>MPGIMKNKKLLCSVCFLFAFMSALWGQNITVKGNVTSKTDGQPIIGASVVETTATTNGTITDFDGNFTLSVPVNSTLKITYIGYKPVTVKAAAIVNVLLEEDTQMVDEVVVTGYTTQRKADLTGAVSVVKVDEIQKQGENNPVKALQGRVPGMNITADGNPSGSATVRIRGIGTLNNNDPLYIIDGVPTKAGMHELNGNDIESIQVLKDAASASIYGSRAANGVIIITTKQGKKGQIKINFDASVSASMYQSKMNVLNTEQYGRAMWQAYVNDGENPNGNALGYAYNWGYNADGNPVLYGMTLSKYLDSKNTMPVADTDWFDEITRTGVIQQYNLSVSNGSEKGSSFFSLGYYKNLGVIKDTDFDRFSARMNSDYKLIDDILTIGQHFTLNRTSEVQAPGGIIETALDIPSAIPVYASDGSWGGPVGGWPDRRNPRAVLEYNKDNRYTYWRMFGDAYVNLTPFKGFNLRSTFGLDYANKQARYFTYPYQEGTQTNNGKSAVEAKQEHWTKWMWNAIATYQLEVGKHRGDVMIGMELNREDDSHFSGYKEDFSILTPDYMWPDAGSGTAQAYGAGEGYSLVSFFGKMNYSYADRYLLSLTLRRDGSSRFGKNHRYATFPSVSLGWRITQENFMKELTWLDDLKLRASWGQTGNQEISNLARYTIYAPNYGTTDSFGGQSYGTAYDITGSNGGGVLPSGFKRNQIGNDNIKWETTTQTNVGIDFSLFKQSLYGSLEYYYKKATDILTEMAGVGVLGEGGSRWINSGAMKNQGFEFNLGYRNKTAFGLTYDLNGNISTYRNEILELPETVAANGKFGGNGVKSVVGHTYGAQVGYIADGIFKSQDEVDNHATQEGAAVGRIRYRDIDHNGVIDERDQNWIYDPTPSFSYGLNIYLEYKNFDLTMFWQGVQGVDIISDVKKKSDFWSASNVGFLNKGTRLLNAWSPTNPNSDIPALTRSDTNNEQRVSTYFVENGSFLKLRNIQLGYTVPAVISKKMRMDRLRFYCSAQNLLTIKSKNFTGEDPENPNFSYPIPVNITFGLNIGF[2x];>[2x]MKKIIYIATIGITLLTTSCDDFLDRQVPQGIVTGDQIASPEYVDNLVISAYAIWATGDDINSSFSLWNYDVRSDDCYKGGSGTEDGGVFNALEISKGINTTDWNINDIWKRLYQCITRANTALQSLDQMDEKTYPLKNQRIAEMRFLRGHAHFMLKQLFKKIVIVNDENMEPDAYNELSNTTYTNDEQWQKIADDFQFAYDNLPEVQIEKGRPAQAAAAAYLAKTYLYKAYRQDGADNALTGINEEDLKQVVKYTDPLIMAKGGYGLETDYSMNFLPQYENGAESVWAIQYSINDGTYNGNLNWGMGLTTPQILGCCDFHKPSQNLVNAFKTDSQGKPLFSTYDNENYEVATDNVDPRLFHTVGMPGFPYKYNEGYIIQKNDDWSRSKGLYGYYVSLKENVDPDCDCLKKGSYWASSLNHIVIRYADVLLMRAEALIQLNDGRITDAISLINEVRSRAAGSTMLIFNYKEDYGVNFKVTPYDLKAYAQDEAMKMLKWERRVEFGMESSRFFDLVRWGEAKDVINAYYVTEASRCSIYKNAGFTENKNEYLPVPFEQISASNGNYTQNFGW;>MMKNMILPIAFTALIASMTACSDETDPILTQKNWDGTATYFQSSDEHGFSMYYKPQVGFVGAPMPFYDPVAKDFKVMYLQDYRPNPEATYHPIFGVATKDGATYESLGELISCGGRDEQDAAIGTGGTIYNPADKLYYTFYTGNKFKPSSDQNAQVVMVATSPDFKTWTKNRTFYLKGDTYGYDKNDFRDPFLFQTEDGVYHMLIATRKNGKGHIAEFTSADLKEWESAGTFMTMMWDRFYECPDVFKMGDWWYLIYSEQASFMRKVQYFKGRTLEDLKATTANDAGIWPDNREGMLDSRAFYAGKTASDGTNRYIWGWCPTRAGNDNGNVGDVEPEWAGNLVAQRLIQHEDGTLTLGVPDAIDRKYTSAQEVKVMAKDGNMIESGKTYTLGEGASVIFNRLKVHNKISFTVKTASNTDRFGISFVRGTDSASWYSIHVNADEGKANFEKDGDDAKYLFDNKFNIPADNEYRVTIYSDQSVCVTYINDQLSFTNRIYQMQKNPWSLCCYKGEITVSDVQVSTY[2x];>[2x]MKSIIKQLYTILLVTVACLTVTGCSDDFKSGLRLDGDVWVNSIRLDEYAGTVDYQNKAIVVGVPYDYDITRMVVTEMNLSEGAKASIAIGETIDFSLPVSLTVKNGDVQMSYTITVKRDEAKILTFKLNDTYVGKVDQLSKTISVVVPLTVDITQLKGTFTVTDGATVTPASGSIQDFTNPVTYTATYRSAVTPYVVTVTQGNVIPTAFVGTASSVSLLTSPEEKAAAQWMMDNVSMSEYISFKDVVDGKVDLGKYTAIWWHFHADNGDNPPLPDDAKAAAEKFKVYYQNGGNLLLTRYATFYIANLGIAKDERVPNNSWGGNEDSPEITSAPWSFLITGSESHPLFQDLRWKDGDKSTVYTCDAGYAITNSTAQWHIGTDWGGYDDLNAWRNLTGGIDLAHGGDGAVVIAEFEPRSNSGRTLCIGSGCYDWYGKGVDASADYYHYNVEQMTLNAINYLCKHHHHHH

Glycan uptake across the bacterial outer membrane (OM) of these bacteria is mediated by SusCD protein complexes, comprising a membrane-embedded barrel and a lipoprotein lid, that is thought to open and close to facilitate substrate binding and transport. Here we show that for both the levan and dextran utilisation systems of Bacteroides thetaiotaomicron, the additional OM components assemble on the core SusCD transporter, forming stable glycan utilising machines which we term ‘utilisomes’. Transport-competent FOS are generated from levan by a surface-exposed lipoprotein, a GH32-family levan endo-glycanase (GHlev), while an SGBP (SGBPlev) is thought to recruit levan at the cell surface. Single particle cryogenic electron microscopy (cryoEM) structures in the absence and presence of substrate reveal concerted conformational changes that demonstrate the mechanism of substrate capture, and rationalise the role of each component in the utilisome.

We reasoned that in a utilisome containing a catalytically inactive GHlev (with the active site D42A mutation), and longer FOS chains (~DP 15-25), the binding of a single levan chain by both GHlev and SGBPlev might reduce conformational variability. We therefore collected such a "long-FOS" cryoEM dataset, and observed in 3D classification that a novel conformation was present, in which the C-terminal domain of SGBPlev adopted a ‘docked’ state proximal to both SusDlev and GHlev (ED Fig. 3c.). The unmasked versions of those 29k particles were then used to generate a final reconstruction of the complete utilisome at 3.0 Å with well-resolved density for a complete SGBPlev. SGBPlev is organised into three domains, as predicted by Alphafold. In addition, density is present at two additional sites that are unique to this long FOS structure. Within the inactivated GHlev active site, there is density for ~five β2,6-linked fructose units, and we define this site as FOS3. A secondary or ‘tethering’ site of FOS binding is also observed (FOS4) with density for FOS bridging between SGBPlev and GHlev. The long, bridging levan molecule binds to GHlev across the top of the GHlev β-propeller domain, before proceeding towards its C-terminal β-sandwich domain. Whilst the resolution is in the region of the bridging levan is insufficient for a detailed description of binding such as hydrogen bonds (3.5-4.0 Å), several tryptophan residues are clearly involved, including W297 and W359 from SGBPlev, and W217 from GHlev, which appear to cradle the levan chain via stacking interactions. The utilisome structure suggests why SusCD transporters exist as dimers. The SGBPlev is clearly inherently flexible, and in the dataset with inactive GHlev and long FOS, a novel conformation was observed in which an untethered SGBPlev from one SusClev contacts the tethered SGBPlev associated with the other SusClev (ED Fig. 4e).> GDVEEAIERAVVHVADTMRSGPSNSASVPALTAVETGHTSQVTPSDTMQTRHVKNYHSRSESTVENFLGRSACVYMEEYKTTDNDVNKKFVAWPINTKQMVQMRRKLEMFTYLRFDMEVTFVITSRQDPGTTLAQDMPVLTHQIMYVPPGGPIPAKVDDYAWQTSTNPSIFWTEGNAPARMSIPFISIGNAYSNFYDGWSNFDQRGSYGYNTLNNLGHIYVRHVSGSSPHPITSTIRVYFKPKHT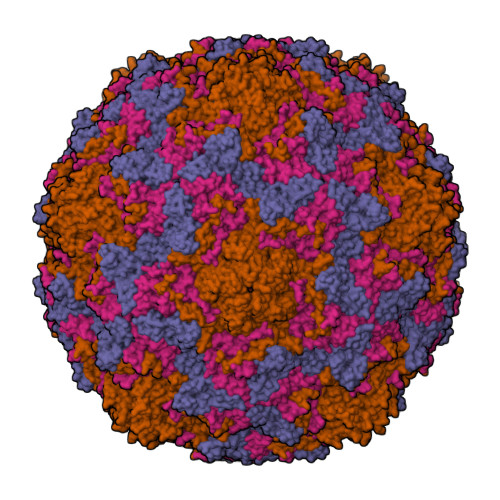RAWVPRPPRLCQYKKAFSVDFTPTPITDTRKDINTVTTVAQSRRRGDMSTLNTH;> SPTVEECGYSDRVRSITLGNSTITTQECANVVVGYGRWPTYLRDDEATAEDQPTQPDVATCRFYTLDSIKWEKGSVGWWWKFPEALSDMGLFGQNMQYHYLGRAGYTIHVQCNASKFHQGCLLVVCVPEAEMGGAVVGQAFSATAMANGDKAYEFTSATQSDQTKVQTAIHNAGMGVGVGNLTIYPHQWINLRTNNSATIVMPYINSVPMDNMFRHYNFTLMVIPFVKLDYADTASTYVPITVTVAPMCAEYNGLRLAQAQ;> GLPTMNTPGSTQFLTSDDFQSPCALPQFDVTPSMNIPGEVKNLMEIAEVDSVVPVNNVQDTTDQMEMFRIPVTINAPLQQQVFGLRLQPGLDSVFKHTLLGEILNYYAHWSGSMKLTFVFCGSAMATGKFLIAYSPPGANPPKTRKDAMLGTHIIWDIGLQSSCVLCVPWISQTHYRLVQQDEYTSAGYVTCWYQTGMIVPPGTPNSSSIMCFASACNDFSVRMLRDTPFISQDNKLQ;> GAQVSTQKTGAHETSLSAAGNSIIHYTNINYYKDAASNSANRQDFTQDPSKFTEPVKDVMIKSLPALN Hosieine | 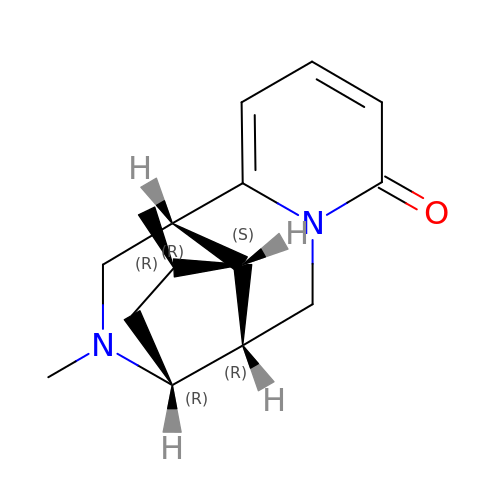C15 H20 N2 O | PDPSDBUFNKLMBE-FPVNZWGXSA-N> GSKPMEVYVSAVASPTKFWVQLIGPQSKKLASMVQEMTSYYSSAENRAKHVLTAPYVGQIVAAVFKFDEKWYRAEIVDIMPNQYNPKEQVIDLYFVDYGDSEYISPADICELRTDFLTLRFQAVECFLANVKSTIQTEPITWPKSSIAKFEELTEVAHWRKLIARVVTYKERPRATTAVS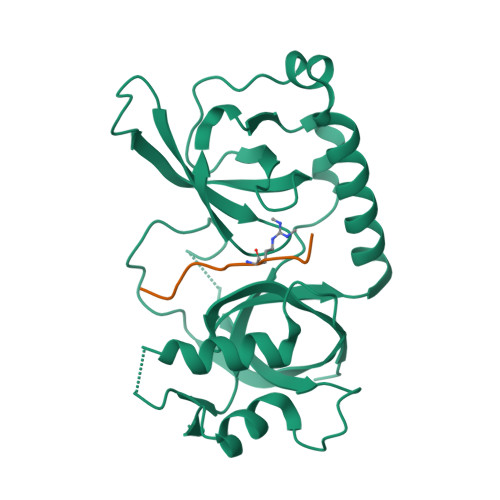AAAKEGTPLPGVELFDPADNSELNIADLMITQGFALPLDDSYP;> DQGRGRRRPLN> PPGPPGP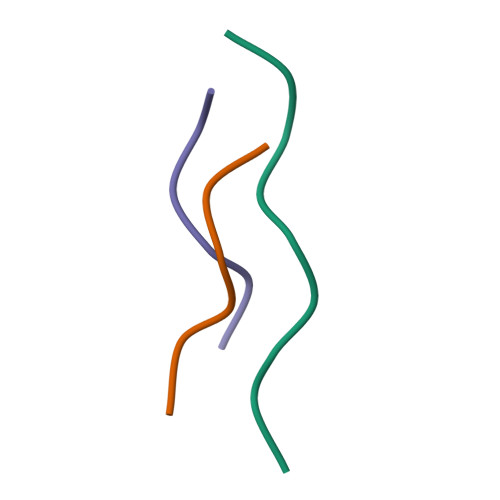PG;>[2x]PPGPPG(2~{S})-2-[[(2~{S})-4-methyl-1-oxidanyl-1-oxidanylidene-pentan-2-yl]carbamoylamino]pentanedioic acid | C12 H20 N2 O7 | 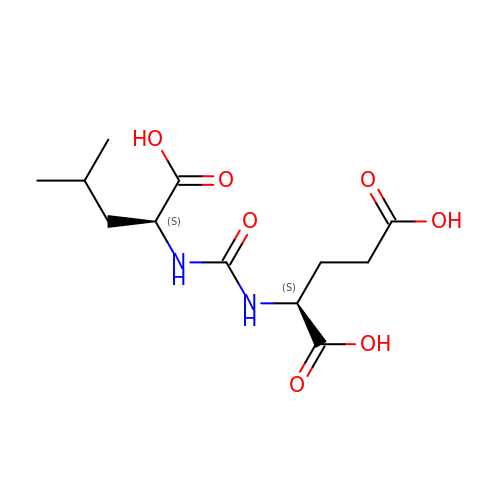BSGWCSGMXAVYRT-YUMQZZPRSA-N>[2x]XXCUCCUAGUACGAGAGGACCGGA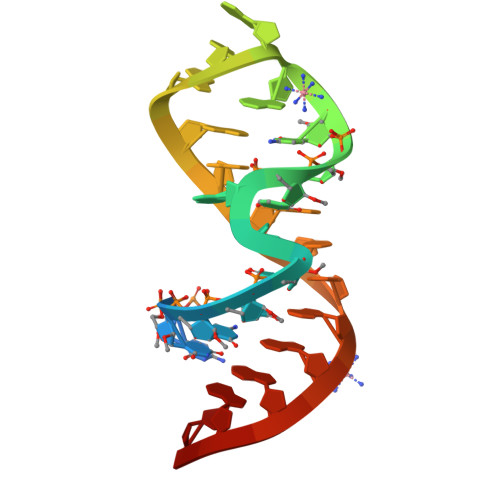GUG> GPLQVSNARLLFPISMPEDEGVVRLVVNNTDESDLQVAVVSLPSFVSLDDRAFRLQAREPRELNLSLAVPRNMPPGMKDEPLVLEVTSPETGKKAVDSVMVSLPLVDNFPALTAAQTGVMELSTYLDMGQLDGETTKAAIEIRNVGAGPLRLHSVTTRNPALTAVPDRTEIKPGGSTLLRIAVDPQVMKAEGWQSIAADISIICNDPQAP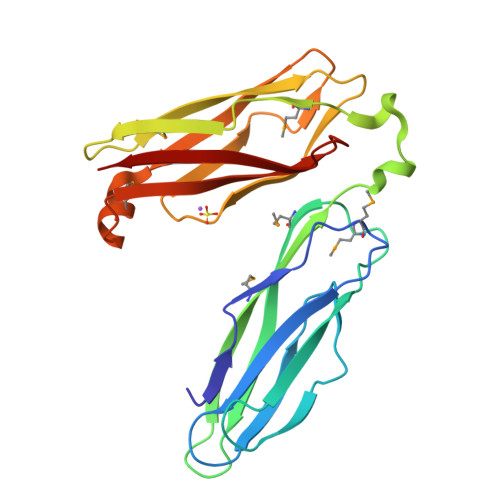LRRIKVKAEL>MHKVSATLLIIDDDEVVRESLAAYLEDSNFKVLQALNGLQGLQIFESEQPDLVICDLRMPQIDGLELIRRIRQTASETPIIVLSGAGVMSDAVEALRLGAADYLIKPLEDLAVLEHSVRRALDRAYLRVENQRYRDKLEAANRELQASLNLLQEDQNAGRQVQMNMLPVTPWSIEGLEFSHRIIPSLYLSGDFVDYFRVDERRVAFYLADVSGHGASSAFVTVLLKFMTTRLLYESRRNGTLPEFKPSEVLAHINRGLINTKLGKHVTMLGGVIDLEKNSLTYSIGGHLPLPVLFVEGQAGYLEGRGLPVGLFDDATYDDRVME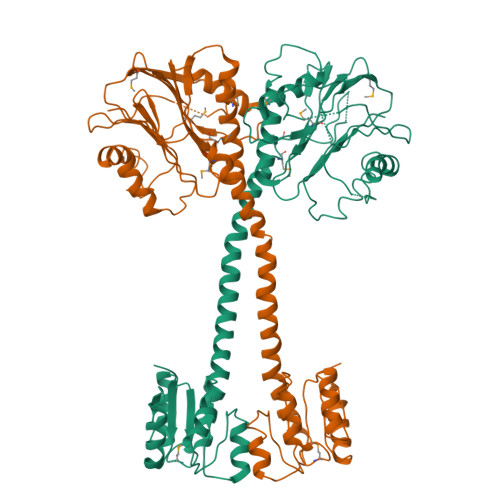LPPSFSLSLFSDGILDVLPGATLKEKEASLPEQVAAAGGTLDGLRQVFGLANLAEMPDDIALLVLSRNLA[2x]>[2x]MVYQVKDQEDFTKQLNEAGNKLVVIDFYATWCGPCKMIAPKLEELSQSMSDVVFLKVDVDECEDIAQDNQIACMPTFLFMKNGQKLDSLSGANYDKLLELVEKNK

Litopenaeus vannamei thioredoxin (LvTrx) is a redox protein with a molecular weight of 12 kDa, which catalyzes the reduction of the disulfide bond in different biological systems. The determination of the crystal structures of LvTrx under different redox conditions discloses a dimeric form mediated by a disulfide bond and other residues that are involved in the dimeric interface. The LvTrx contains four cysteines; two of them are engaged to form a catalytic disulfide bond (Cys32 and Cys35); Cys62 is not involved in any interactions, but in human thioredoxin (hTrx), it has been reported that Cys62 is readily S-nitrosylated, giving a SNO modification; and Cys73, which in previous studies, showed a dimeric behavior in the crystal system of hTrx and LvTrx, mediated by the interface disulfide bond through the Cys73 residue of each monomer. In an attempt to determine if the interface disulfide bond is viable to be reduced or if it is a consequence of a crystalline arrangement, we used X-rays as a tool to conduct experiments of radiation damage to monitor the reduction of the interface disulfide bond in two crystals of LvTrx.

During data collection, two crystal of LvTrx were diffracted at different transmissions, referred to below as LvTrx-1x (8% of transmission, 1.33 × 10 11 photons·s−1) and LvTrx-3x (27% of transmission, 4.14 × 1011 photons·s−1). Ten datasets were collected for each crystal, with the purpose of analyzing the sequential increase in the absorbed dose of energy. Specifically, changes were observed in the electron density corresponding to the region of the interface disulfide bond (Cys73-Cys73') and the catalytic disulfide bond (Cys32-Cys35) of each monomer. The deterioration of the electron density was dependent on the increment of the absorbed dose. In the case of the crystal LvTrx-1x, the interface disulfide bond (Cys73-Cys73') remained stable, reaching a dose of 34 MGy. However, at a dose of 3.4 MGy, this disulfide bond showed double conformations in the Sγ atoms of the residues Cys73-Cys73' without compromising the disulfide bond formation. The interface disulfide bond is shown as one of the most stable disulfide bonds to our knowledge, even with a significant solvent exposure.> MRALIIVDVQNDFCEGGSLAVTGGAALARAISDYLAEAADYHHVVATKDFHIDPGDHFSGTPDYSSSWPPHCVSGTPGADFHPSLDTSAIEAVFYKGAYTGAYSGFEGVDENGTPLLNWLRQRGVDEVDVVGIATDHCVRQTAEDAVRNGLAT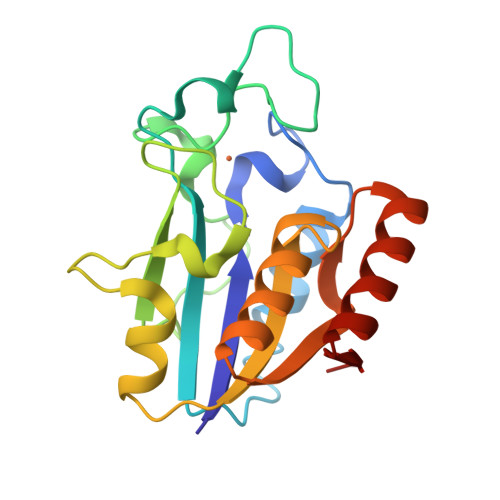RVLVDLTAGVSADTTVAALEEMRTASVELVCSS Ferritins are proteins forming 24meric rhombic dodecahedral cages that play a key role in iron storage and detoxification in all cell types. Their function requires the transport of Fe2+ from the exterior of the protein to buried di-iron catalytic sites, known as ferroxidase centres, where Fe2+ is oxidized to form Fe3+-oxo precursors of the ferritin mineral core. SynFtn, isolated from the cyanobacterium Synechococcus CC9311, is an atypical prokaryotic ferritin that was recently shown to take up Fe2+ via its threefold channels. The wild-type protein contains three iron binding sites: high- and low-affinity binding sites at the FOC, sites 1 and 2, respectively, and site 3 located in the threefold channel and coordinated by the side chains of three symmetry equivalent Asp137 residues.

Crystal structures of SynFtn have been reported in the iron-free state and following either 2 or 20 min of soaking in a 5 mm Fe2+ solution. These revealed conformational flexibility of the side chain of residue Glu141, which is located close to the inner surface exit of the threefold channel. To probe the possibility that Glu141 of SynFtn acts as a ‘transfer’ carboxylate with equivalent function to the conserved carboxylates of the animal ferritins, two variants, E141A and E141D, were generated. Variants E141A and E141D both crystallized under conditions identical to those reported for wild-type SynFtn. Protein structures derived from all crystals harvested without iron enrichment were free of bound metal ions, as expected. The structures of variants E141A and E141D overlay with that reported for the wild-type protein with overall rmsd (for main chain atoms) of 0.10 and 0.11 Å, respectively, with the major difference in structure being associated with the side chain of the substituted residue. Typically when site 3 is vacant, residue 141 is oriented toward the FOC. This is the case for the metal-free structure of variant E141D, while conformational flexibility at this position is not possible in E141A. In the case of E141A the second-order rate constant extracted from the gradient of this plot was 1.1×105  m −1 s−1, significantly lower than that measured for wild-type SynFtn. The data reported here demonstrates that transport of iron to the FOC is inhibited in SynFtn variant E141A. However, the effect is less severe than that caused by disruption of the threefold channel by the D137A substitution that led to loss of all rapid Fe2+ oxidation activity. This suggests that residue Glu141 is not essential for Fe2+ to traverse the protein coat, and that its role is to direct incoming metal toward the catalytic FOCs.

> MATDVAQGPNGRALAESMNPDLLSAIQQHISIERYASVTYLAMSIWCAERELAGFYQFFDGEAKDEQSHAVHFTQYLIARSQSNDLQTLDAPRQNWDSLASLMATAFQMEADTTSSIQSVYALAERNSDTRTTVFLDPLIAAQIQSEDQFAYLLGRVKFANGDPTALLVIDNELRAGQTQRG> MAPSRANTSVIVVGGGGTIGSSTALHLVRSGYTPSNVTVLDAYPIPSSQSAGNDLNKIMGVSLRNPVDLQLALEARQMWNEDELFKKFFHNTGRLDCAHGEKDIADLKSGYQALVDAGLDATNEWLDSEDEILKRMPLLSRDQIKGWKAIFSKDGGWLAAAKAINAVGEYLRDQGVRFGFYGAGSFKAPLLAEGVCIGVETVDGTRYYADKVVLAAGAWSPTLVELHEQCVSKAWVYGHIQLTPEEAARYKNSPVVYNGDVGFFFEPNEHGVIKVCDEFPGFTRFKMHQPFGAKAPKRISVPRSHAKHPTDTIPDASDVSIRRAIATFMPQFKNKKMFNQAMCWCTDTADAALLICEHPEWKNFVLATGDSGHSFKLLPNIGKHVVELLEGTLADDLAHAWRWRPGSGDALKSRRSAPAKDLADMPGWNHDKPRANLLEHHHHHH

N-valyl-histidine derived from proteolytic digestion of the N-terminus of the HbA1c β-chain. This study reports the X-ray structures of the wild-type and Asn56Ala (N56A) mutant of Phaeosphaeria nodorum fructosyl peptide oxidase (PnFPOX) to elucidate the residues responsible for the oxidative half-reaction. Fructosyl amine oxidases (FAOXs) are FAD-containing enzymes that catalyze the oxidative deglycosylation of fructosyl amino acids such as fructosyl valine and/or ε-fructosyl lysine, which are the degradation products of HbA1c and GA, respectively. As members of the FAOX family, fructosyl peptide oxidases (FPOXs) are also known as candidates for diagnostic enzymes. A covalent bond is formed between FAD and Cys343 of PnFPOX as observed in amadoriase I (Cys342), amadoriase II (Cys335), and EtFPOX (Cys347).

A bound acetate to wild-type PnFPOX is located at the re-face of the isoalloxazine ring of FAD. The bound acetate of wild-type PnFPOX corresponds to the position of bound beta-D-fructopyranose (BDF) in amadoriase I and the position of FSA in amadoriase II. The positions of the O1, O2, and CH3 of the bound acetate correspond to the O5, C4, and C6, respectively, of the bound BDF and the fructosyl moiety of the bound FSA. This suggests that the position of the bound acetate is the binding site of a region of the fructosyl moiety of the substrate (fructosyl amino acids). In wild-type PnFPOX, Asn56 forms a hydrogen bond with Lys274; Lys274 forms water (W1)-mediated hydrogen bonds with N5 of FAD and hydrogen bonds with Asp54 and Lys57 and O2 of FAD via a water molecule (W2). The direct distance between Lys274 and Asp54 is 5.48–6.03 Å in wild-type PnFPOX. In wild-type PnFPOX, Asn56 forms a hydrogen bond with Lys274 (2.93 Å), which interacts with N5 of the isoalloxazine ring of FAD by a water-mediated hydrogen bond. The water molecule (W1) is located at the si-face of the isoalloxazine ring 2.51 Å from Lys274 and 3.22 Å from N5 of the isoalloxazine ring. Interestingly, the related positions of Lys57 and W2 in wild-type PnFPOX correspond to those of Arg49 and the bound chloride in MSOX, suggesting that the W2 position might be a putative oxygen-binding site in PnFPOX. The analysis of the protein channels of the structures showed that the W1, W2, and W4 positions in wild-type PnFPOX (W1′ and W4′ in PnFPOX N56A) are in the main oxygen-accessible channel. The positions of the side chains of Ser62, Arg64, Arg94 and His373 create a smaller cavity for accepting and recognizing substrates in PnFPOX compared to EtFPOX.>MLTQHVSEARTRGAIHTARLIHTSDLDQETRDGARRMVIEAFRDPSGDSDFTDDFTDDDWDHALGGMHALISHHGALIAHGAVVQRRLMYRGPDGRGHALRCGYVEAVAVREDRRGDGLGTAVLDALEQVIRGAYQIGALSASDIARPMYIARGWL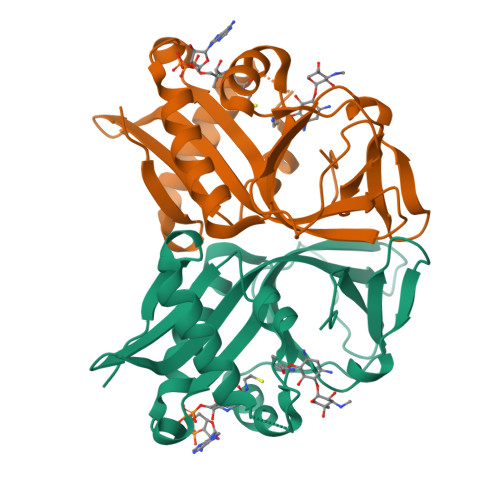SWEGPTSVLTPTEGIVRTPEDDRSLFVLPVDLPDGLELDTAREITCDWRSGDPW[2x]>MKHELPPLPYAYNALEPFIDAKTLEIHHTKHHQSYVDKLNAALEKYPDLQDKTVEELIKSLNELPEEIRTTVRNNAGGHFSHTLYWNIMNPATQEYIPEELGNALVETFGSIIAFKEQFSKAAANIFGSGWVWLAADANKKLKIVSTTGHDNPLMTGDAPLMVIDIWEHAYYLHYQNRRPEYIENWWNVLDWKAVEERYNALG[2x]

Here we studied metal-preference evolution within the natural diversity of the iron/manganese superoxide dismutase (SodFM) family of reactive oxygen species scavengers. Only a few metalloenzymes have been rigorously demonstrated to be cambialistic in vivo, including some iron (Fe)- or manganese (Mn)-dependent superoxide dismutases (SODs; SodFMs); metalloenzymes that play an important role in cellular reactive oxygen species defence. To study this process, we leveraged the existence of naturally Fe-specific, Mn-specific and flexible Fe/Mn-cambialistic SodFM homologues, which differentially utilize these metals to catalyse the detoxification of superoxide. By combining phylogenetics, biochemistry and structural biology, we demonstrate that SodFM metal utilization can be evolutionarily fine tuned by sliding along a scale between perfect manganese and iron specificities.

CPR Wolfebacteria represented a striking and highly unusual emergence of dimeric Fe-preferring SodFM1 containing SodFM3/4-like HCterm and VD-2 residues. SodFM1s and SodFM4s were found in uncultured CPR Wolfebacteria (c). Although SodFMs are a well-studied protein family, with over 50 WT protein crystal structures available from various organisms, we were able to uncover additional diversity via application of bioinformatics and phylogenetics on a dataset of genomes sampled across the tree of life. This included the novel categorization of the SodFM protein family into five distinct subfamilies, the first comparison of multiple members of the largely unstudied group of SodFM4s, and identification of atypical isozymes such as the Fe-preferring SodFM1 from CPR Wolfebacterium. In some cases, such as Nesterenkonia alba SodFM3 Q/H, a single residue has a major impact on the preferred metal co-factor, while in others, such as CPR SodFM1 H/Q, mutation at the same position had a negligible effect. Importantly, consistent with previous reports, comparison of four protein crystal structures of the WT and mutant SodFMs we determined here indicated that metal-preference modulation by XD-2 and Q/H occurs without any significant changes to the secondary metal coordination sphere within the resolution limits of the solved structures.>[4x]DSESDCTGSEPVDAFQAFSEGKEAYVLVRSTDPKARDCLKGEPAGEKQDNTLPVMMTFKNGTDWASTDWTFTLDGAKVTATLGNLTQN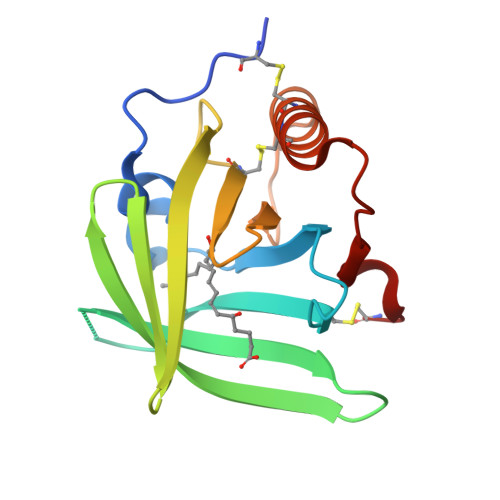REVVYDSQSHHCHVDKVEKEVPDYEMWMLDAGGLEVEVECCRQKLEELASGRNQMYPHLKDC> EMSVKPTAPQDKSVPVWNGFSLYTDDTVKAAAQYAYDNYLGKPYTGSVESAPANFGGRMVYRQHHGLSHTLRTMAYAELIVEEARKAKLRGETLGKFKDGRTIADVTPQELKKIMIAQAFFVAGRDDEASDAKNYQKYHEQSRDAFLKYVKDNESTLIPDVFKDQEDVNFYARVIEDKSHDWESTPAHVLINQGHMVDLVRVKQPPESFLQRYFSSMQRWIGSQATEAVFGIQRQFFHATYEVVAGFDSDNKEPHLVVSGLGRYVIGEDGQPIREAPKKGQKEGDLKVFPQTYKLKENERLMRVDEFLKLPEIQNTFPGSGKHLQGGMPGMNEMDYWNRLNSLNRARCENDVDFCLKQLQTAHDKAKIEPIKQAFQSSKG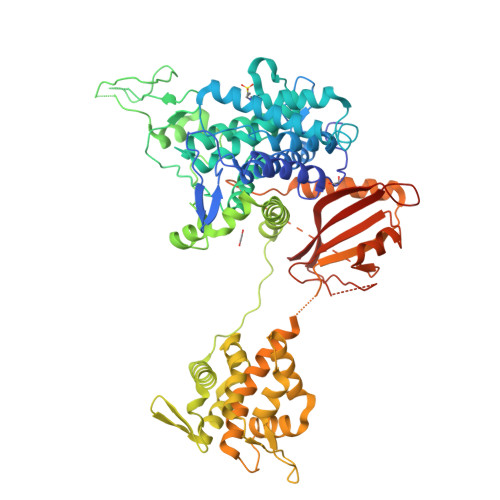KERRQPNVDEIAAARIIQQILANPDCIHDDHVLINGQKLEQQFFRDLLAKCEMAVVGSLLNDTDIGNIDTLMRHEKDTEFHSTNPEAVPVKIGEYWINDQRINNSSGNITQKKHDLIFLMQNDAWYFSRVNAIAQNRDKGSTFKEVLITTLMTPLTSKALVDTSQAKPPTRLFRGLNLSEEFTKGLIDQANAMIANTTERLFTDHSPEAFKQIKLNDLSKMSGRTNASTTTEIKLVKETWDSNVIFEMLDPDGLLHSKQVGRHGEGTESEFSVYLPEDVALVPVKVTLDGKTQKGENRYVFTFVAVKSPDFTPRH> GAMGSRKSKAELQSEERKRIDELIESGKEEGMKIDLIDGKGRGVIATKQFSRGDFVVEFHGDLIEITDAKKREALYAQDPSTGCYMYYFQYLSKTYCVDATRETNRLGRLINHSKCGNCQTKLHDIDGVPHLILIASRDI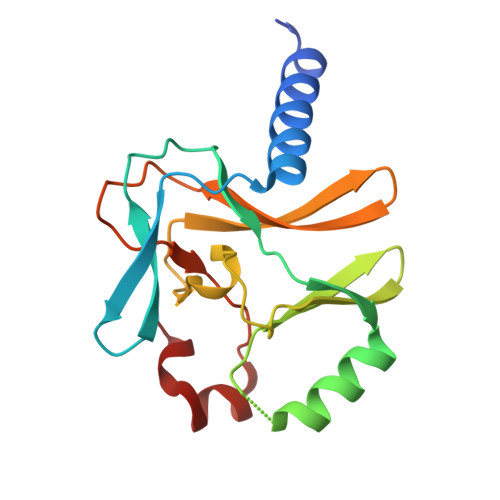AAGEELLYDYGDRSKASIEAHPWLKH> MGHHHHHHMSHTILLVQPTKRPEGRTYADYESVNECMEGVCKMYEEHLK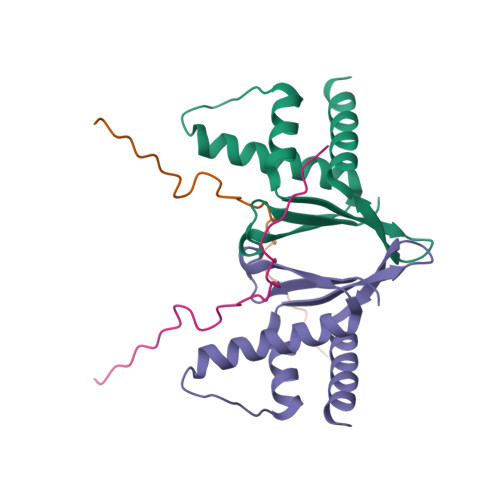RMNPNSPSITYDISQLFDFIDDLADLSCLVYRADTQTYQPYNKDWIKEKIYVLLRRQAQQAGK;> PRTARHAPAVRKFSPDLKLLKDVKISVSFTE>MGHHHHHHMTKIKWLGAFALVFVMLLGGCSLPGLGGASDDTIKIGAQSMTESEIVANMIAQLIEHDTDLNTALVKNLGSNYVQHQAMLGGDIDISATRYSGTDLTSTLGKEAEKDPKKA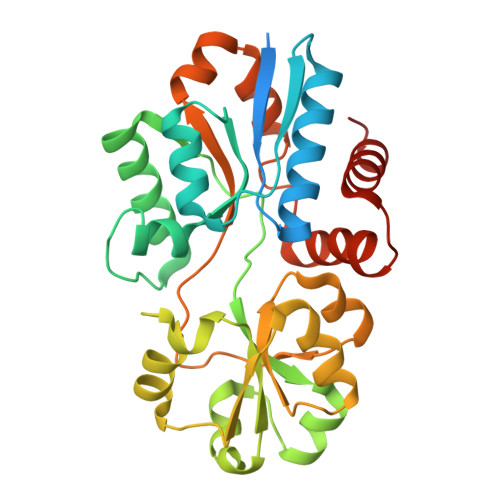LNIVQNEFQKRFSYKWFDSYGFDNTYAFTVTKKFAEKEHINTVSDLKKNASQYKLGVDNAWLKRKGDGYKGFVSTYGFEFGTTYPMQIGLVYDAVKNGKMDAVLAYSTDGRIKAYDLKILKDDKRFFPPYDCSPVIPEKVLKEHPELEGVINKLIGQIDTETMQELNYEVDGKLKEPSVVAKEFLEKHHYFD[2x]> KG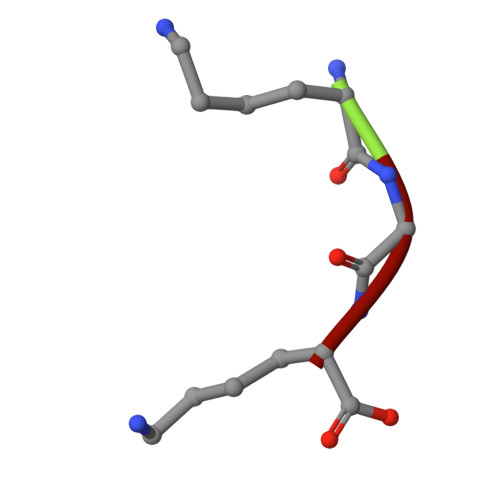K> MHGRLKVKTSEEQAEAKRLEREQKLKLYQSATQAVFQKRQAG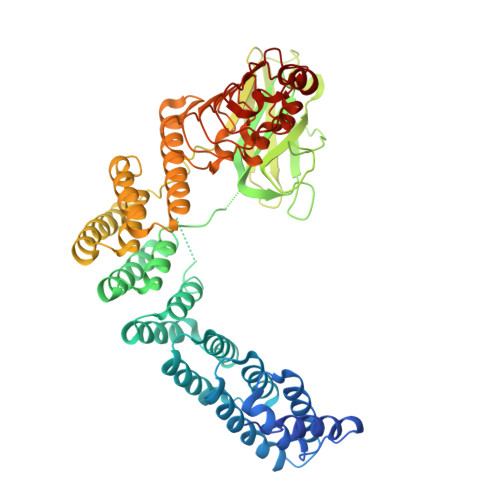ELDESVLELTSQILGANPDFATLWNCRREVLQHLETEKSPEESAALVKAELGFLESCLRVNPKSYGTWHHRCWLLSRLPEPNWARELELCARFLEADERNFHCWDYRRFVAAQAAVAPAEELAFTDSLITRNFSNYSSWHYRSCLLPQLHPQPDSGPQGRLPENVLLKELELVQNAFFTDPNDQSAWFYHRWLLGRAEPHDVLCCVHVSREEACLSVCFSRPLTVGSRMGTLLLMVDEAPLSVEWRTPDGRNRPSHVWLCDLPAASLNDQLPQHTFRVIWTGSDSQKECVLLKDRPECWCRDSATDEQLFRCELSVEKSTVLQSELESCKELQELEPENKWCLLTIILLMRALDPLLYEKETLQYFSTLKAVDPMRAAYLDDLRSKFLLENSVLKMEYADVRVLHLAHKDLTVLCHLEQLLLVTHLDLSHNRLRALPPALAALRCLEVLQASDNALENVDGVANLPRLQELLLCNNRLQQSAAIQPLVSCPRLVLLNLQGNSLCQEEGIQERLAEMLPSVSSILT>[2x]MAKDKEFQVLFVLTILTLISGTIFYST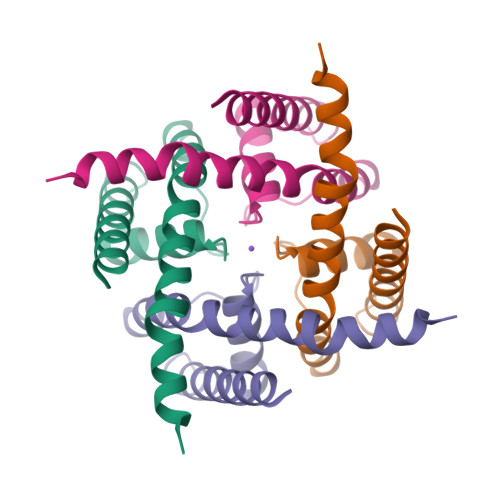VEGLRPIDALYFSVVTLTTVGYGNFSPQTDFGKIFTILYIFIGIGLVFGFIHKLAVNVQLPSILSNLVPR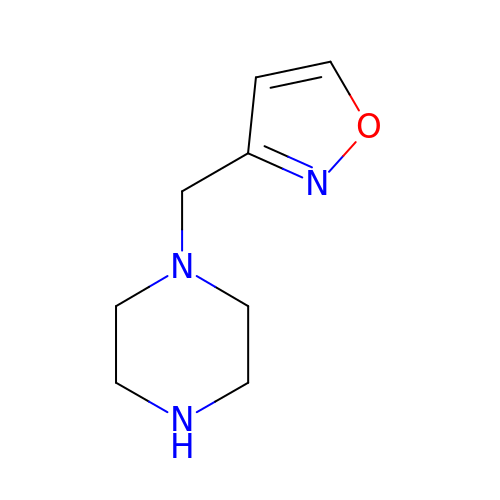1-[(1,2-oxazol-3-yl)methyl]piperazine | C8 H13 N3 O | VJMTXOUUYNPWLF-UHFFFAOYSA-N Inorganic pyrophosphatase (PPase) catalyses the hydrolysis reaction of inorganic pyrophosphate (PPi) to two inorganic phosphates (Pi) and plays an essential role for living organisms. We previously reported the expression and purification of family II PPase from the psychrophilic Shewanella sp. AS-11 (Sh-PPase) isolated from shellfish living in the Southern Ocean (Antarctic Ocean). Sh-PPase activated by Mn2+ ions (Mn-Sh-PPase) displayed the highest activity at 5 °C, which is characteristic of cold-adapted enzymes. X-ray crystallography and EPR spectroscopy were used to investigate a cold-adapted family II Sh-PPase from a psychrophilic bacterium that lives in the Southern Ocean.

In contrast, Sh-PPase activated by Mg2+ ions (Mg-Sh-PPase) has much lower catalytic activity with PPi or PNP than Mn-Sh-PPase13, and we obtained well-diffracted crystals of Mg-Sh-PPase in the presence of PNP and sodium fluoride. X-ray diffraction data at 1.3 Å resolution were obtained. The electron density unambiguously showed that the PNP and four Mg2+ atoms were bound to the di-metal centre of Sh-PPase. In the crystal structure of Mg-Sh-PPase with PNP, the bridged water between Mg2+ ions at M1 and M2 is assumed to be replaced by a fluoride ion. An anomalous difference Fourier map indicated that M1 and M2 metal sites in the crystal structure of Mg-Sh-PPase contain a small fraction of metals other than Mg2+. Based on the anomalous scattering factor of these elements (f ″ = 0.24 for S; f ″ = 1.6 for Fe) at an X-ray wavelength of 1.0 Å, M1 and M2 were occupied by Fe with an estimated content of 15% and 7%, respectively. The M1 site was converted to the 6-coordinated slight rhombic octahedral geometry by binding of PNP, and the M2 site was changed to a nearly axial octahedral coordination sphere. In addition, a bridged water in the crystal structure of Mg-Sh-PPase with PNP, as well as Bs-PPase, shows the formation of unique tri-metal coordination sphere, where it is bound with 3 metal ions (M1, M2 and M4). In fact, the crystal structure of Mg-Sh-PPase with PNP displayed a shorter distance between M1/M2 and the bridged fluoride ion. The overall structure consisted of N- and C-terminal domains, and the overall conformation was changed from the ‘open’ to ‘closed’ state by the binding of substrate, as occurs with other family II PPases.

>MGSMYVVGHKIPDSDSICGAIALAYLKNQIGEPAIAARLGELSPETAFILEKFGFEAPEYKTSYAGEEVYIVDHSEITQAPDDIAQATIVGIVDHHKLGDLTTSTPLECWIRPVGCSNTVIKMMYDFYQVKIPANIAGIMMCAILSDTVIFKSPTCTTADIRCVEALAEIAGVEDFKEVGMDMFKVKSAVEGTPARDLVMRDFKDFNMNGNLVGIGQLEVIDLAVFDDIKADLEADIAKLKVEGNRHSVLLLLTDIMKEGSEMLVVSDSADLTERAYGKPTVDGRVWLDGVLSRKKQVVPALQDAFQKV[2x]> MAHHHHHHSSGLEVLMDAPMEDAPAPVAQVKVIFTTTEPDLELPESKRQLLVPADIRRYGLSRILNSESMLDTGSIPFDFLINGSFLRSSLEDYLTSNGLSLETTLTLQYVRSLIPPVYEASFEHDDWVSAVDVLSATSPAGRWSSAANSSAAVQPGQERVLSASYDGLLRIWNASGSVIATSPSGSHGGHTASIKAAKFLTSDRLASAGMDRTVRVWKYTESDHFTGELKPTLELYGHTGSVDWLDVDGHSKHILTASADGAIGFWSASKASAPEPDASLLPGAHVSKRRKATSSVSTAQRGPLGLWSIHTAPATAAIFDPRDRTVAYSASQDHTVRTLDLTTGQVVSTLTLTHPLLSLSALTRAGTTSPLLAAGTSARHITMVDPRASSATTSVMTLRGHANKVVSLSPSPENEYSLVSGSHDGTCRVWDLRSVRPATKEEGSLGGVSEPVYVIERESWASKGKKKRPVAGDGCKVFSVVWDKLGIFSGGEDKKVQVNRGRNIVTEQK;> PSPDELKPFPTVQQTIFRGHEGRVRSVAIDPTGVALATGGDDGTVRVWELLTGRQVWSVKLNGDEAVNTVRWRPTKDTFILAAAAGEDIFLMIPTHPSVTPALDQASRDILNAGFGHATNGKQQANLPPGKEPPGKWARPGTRLEDEGVLLRITVRSTIKAISWHRRGDHFATVSPSGQRSSVAIHTLSKHLTQIPFRKLNGLAQTA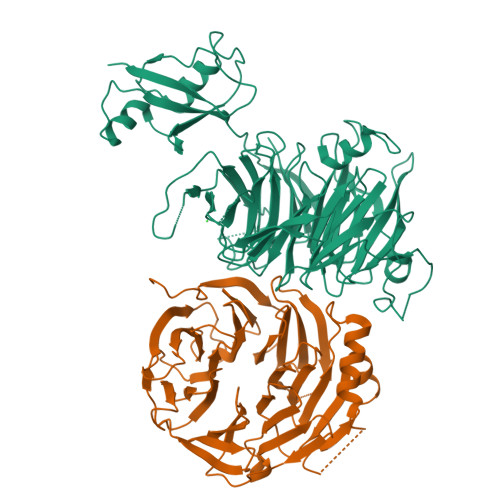SFHPLRPLFFVATQRSIRCYDLQKLELVKIVQPGAKWISSFDVHPGGDNLVVGSYDKRLLWHDLDLSNRPYKTMRFHTEAIRAVRFHKGGLPLFADASDDGSLQIFHGKVPNDQLENPTIVPVKMLKGHKVVNKLGVLDIDWHPREPWCVSAGADGTARLWM>ERLCHPCPWEWTFFQGNCYFMSNSQRNWHDSITACKEVGAQLVVIKSAEEQNFLQLQSSRSNRFTWMGLSDLNQEGTWQWVDGSPLLPS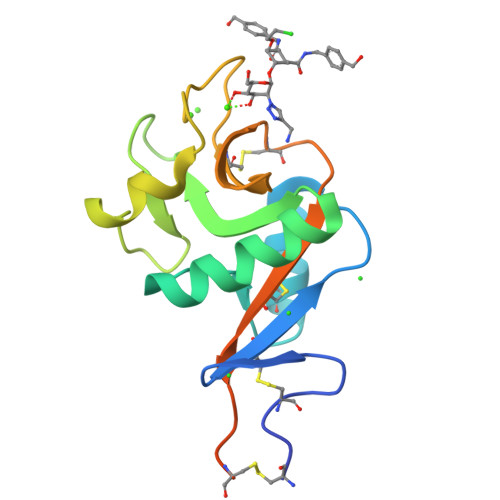FKQYWNRGEPNNVGEEDCAEFSGNGWNDDKCNLAKFWICKKSAASCSRDEEQFLSPAPATPNPPPA[6x]> APVFAAPVTENYVTVQKDWKNTVKKIQEAIKLKSVTSVEVSYNDKSVSTIDLSGKTKVSELEAEAENLYNLVDSKLSNLDDGDSVTFKVTYNTGFNKRFYSKSELEKIKTQLEKKVVVAKGDGKAAGLAMNENGKAVVADRDLVASDFYNFIISTDTSTGEYILKSEKKGAASLDALNEKYGYAALAIDGTGDFGTVTESYVPAAPTDILKSTKQIDETASFENTGKDIAAMTVKAADPGEDGNIANIKVINAKETTIDVDSKSSTSAEDLAKKYVFDDKDLKAVYDQLNEGDGTTGKYVEKVDGRYQVVLYPEGKRLETKS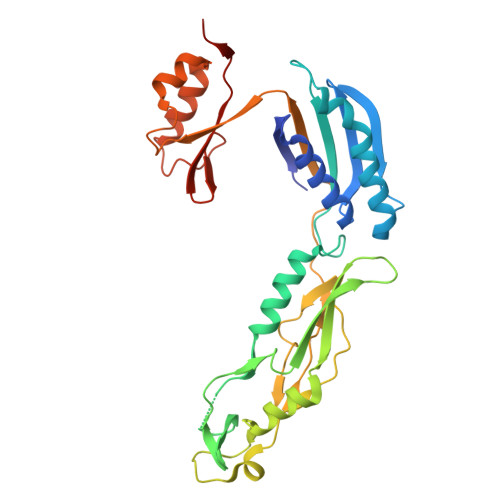AS>[2x]GPGSMSSMKIAIAGASGRMGRML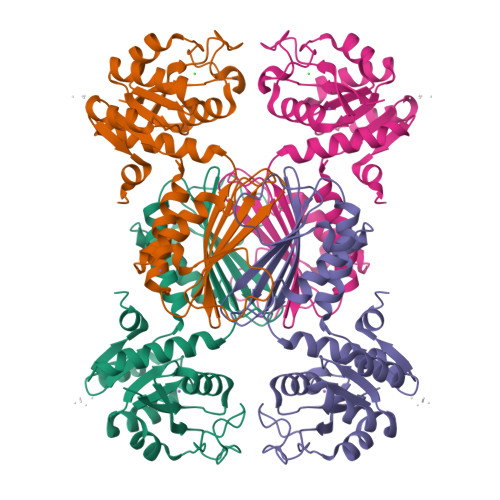IEAVLAAPDATLVGALDRTGSPQLGQDAGAFLGKQTGVALTDDIERVCAEADYLIDFTLPEGTLVHLDAALRHDVKLVIGTTGFSEPQKAQLRAAGEKIALVFSANMSVGVNVTMKLLEFAAKQFAQGYDIEIIEAHHRHKVDAPSGTALMMGETIAAATGRSLDDCAVYGRHGVTGERDPSTIGFSAIRGGDIVGDHTVLFAGIGERIEITHKSASRVSYAQGALRAARFLAGRDAGFFDMQDVLGLR> MTATSDLIESLISYSWDDWQVTRQEARRVIAAIRNDNVPDATIAALDKSGSLIKLFQRVGPPELARSLIASIAGRTTMQRYQARNALIRSLINNPLGTQTDNWIYFPTITFFDICADLADAAGRLGFAAAGATGVASQAIQGPFSGVGATGVNPTDLPSIAFGDQLKLLNKDPATVTKYSNPLGDLGAYLSQLSPQDKLNQAQTLVGQPISTLFPDAYPGNPPSRAKVMSAAARKYDLTPQLIGAIILAEQRDQTRDEDAKDYQAAVSIKSANTSIGLGQVVVSTAIKYELFTDLLGQPVRRGLSRKAVATLLASDEFNIFATARYIRYVANLASQQDLRKLPKT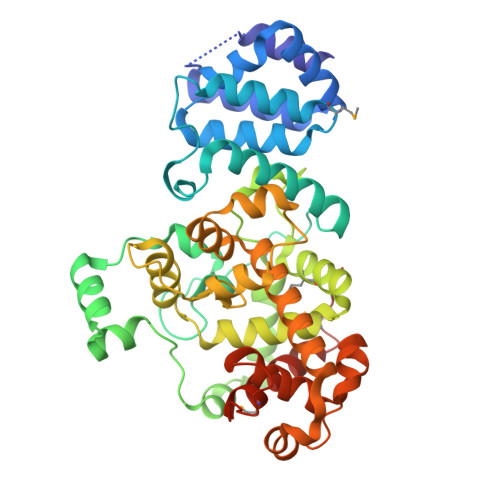RGAFPSIDLRAYAGNPRNWPRDNVRALASEYTSRPWDDNLSPGWPMFVDDAYATFLDPGMRFPLEHHHHHH>AAVILESIFLKRSQQKKKTSPLNFKKRLFLLTVHKLSYYEYDFERGRRGSKKGSIDVEKITCVETVVPEKNPPPERQIPR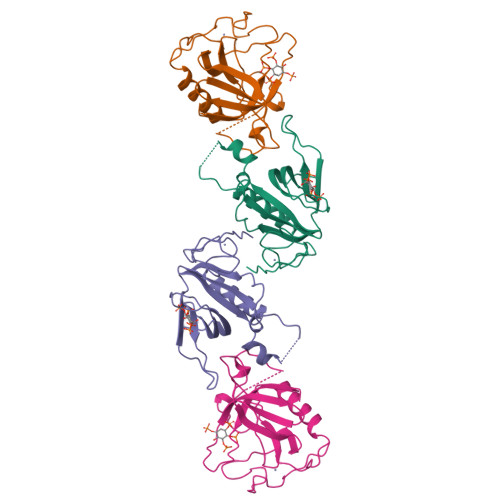RGEESSEMEQISIIERFPYPFQVVYDEGPLYVFSPTEELRKRWIHQLKNVIRYNSDLVQKYHPCFWIDGQYLCCSQTAKNAMGCQILEN[2x]>MAALMTPGTGAPPAPGDFSGEGSQGLPDPSPEPKQLPELIRMKRDGGRLSEADIRGFVAAVVNGSAQGAQIGAMLMAIRLRGMDLEETSVLTQALAQSGQQLEWPEAWRQQLVDKHSTGGVGDKVSLVLAPALAACGCKVPMISGRGLGHTGGTLDKLESIPGFNVIQSPEQMQVLLDQAGCCIVGQSEQLVPADGILYAARDVTATVDSLPLITASILSKKLVEGLSALVVDVKFGGAAVFPNQEQARELAKTLVGVGASLGLRVAAALTAMDKPLGRCVGH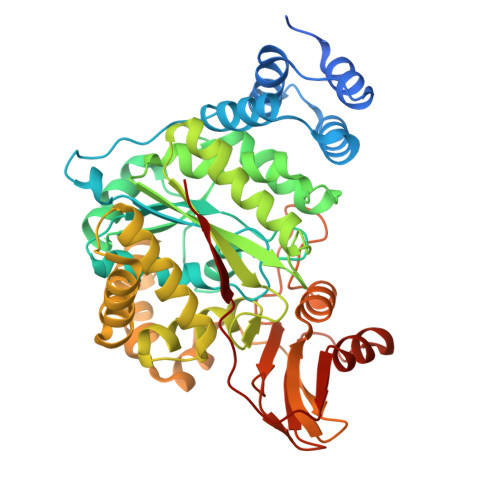ALEVEEALLCMDGAGPPDLRDLVTTLGGALLWLSGHAGTQAQGAARVAAALDDGSALGRFERMLAAQGVDPGLARALCSGSPAERRQLLPRAREQEELLAPADGTVELVRALPLALVLHELGAGRSRAGEPLRLGVGAELLVDVGQRLRRGTPWLRVHRDGPALSGPQSRALQEALVLSDRAPFAAPSPFAELVLPPQQ[4x]> 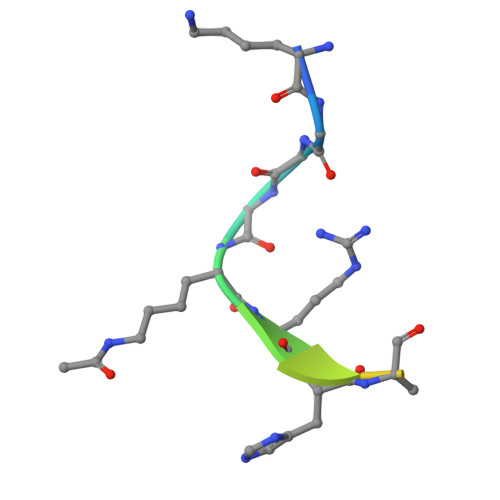KGGAKRHRKILTAQ~{N}-[2-methoxy-5-(oxidanylcarbamoyl)phenyl]dibenzofuran-4-carboxamide 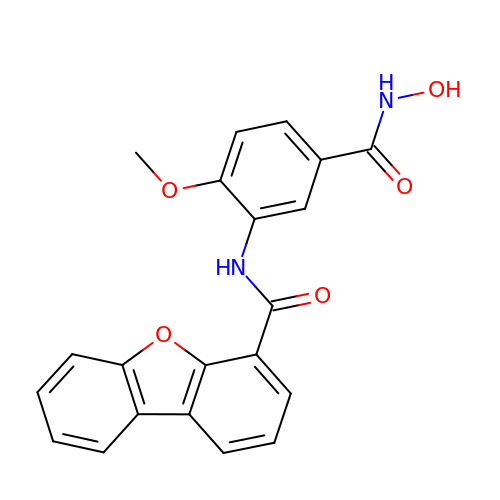| C21 H16 N2 O5 | RFROQVRGDKTHLN-UHFFFAOYSA-N~{S}-(2-acetamidoethyl) (~{E})-oct-2-enethioate 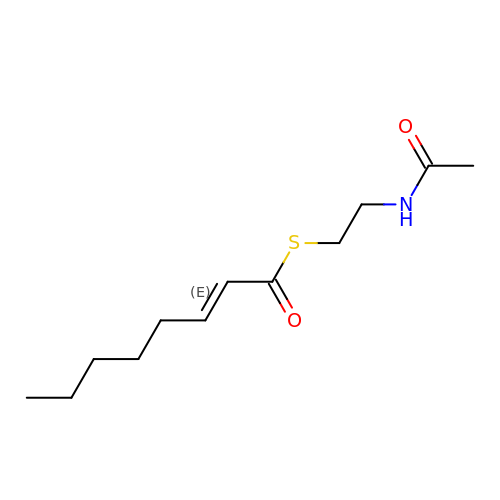| C12 H21 N O2 S | MHEVUMKRTBGSJW-BQYQJAHWSA-N>AAASYDQLLKQVEALKMENSNLRQELEDNSN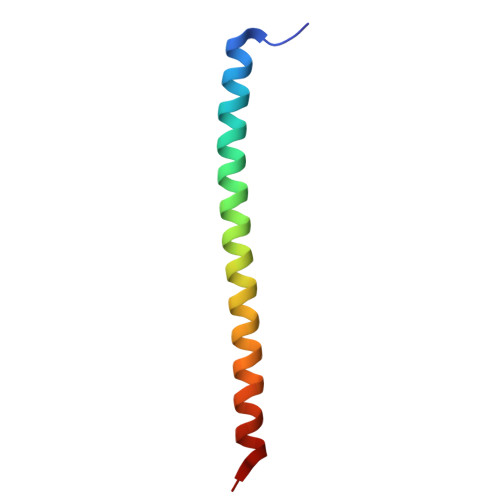HLTKLETEASNMKEVLKQLQGSI[2x]> MSLEEELRRETLKWLERIEERVKEIEGDEGFMRNIEAYISDSRYFLEKGDLVRAFECVV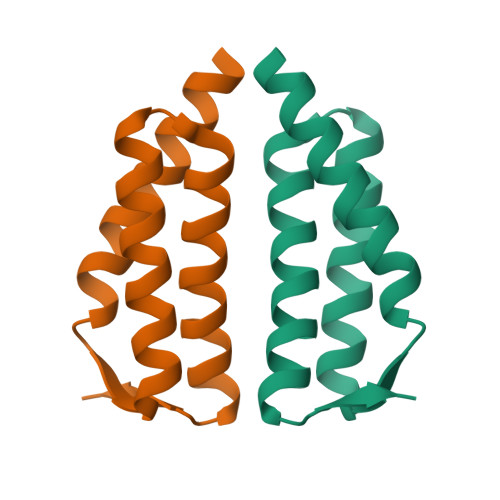WAWAWLEIGLEVGKLHETAEGHHHHHH>[2x]MRPPQFTRAQWFAIQHISLNPPRCTIAM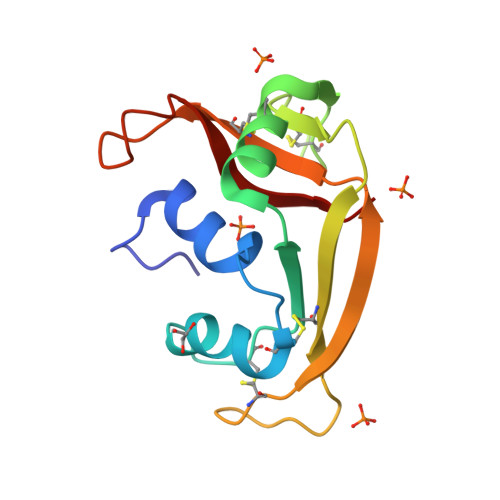RAINNYRWRCKPVNTFVHEPLVDVQNVCFQEKVTCKNGQGNCYRSRFRMHITDCRLTNGSRYPNCRYRTRPGRRHIIVACENRDPRDSPRYPYVPVHFDASV>MSRAAQLLP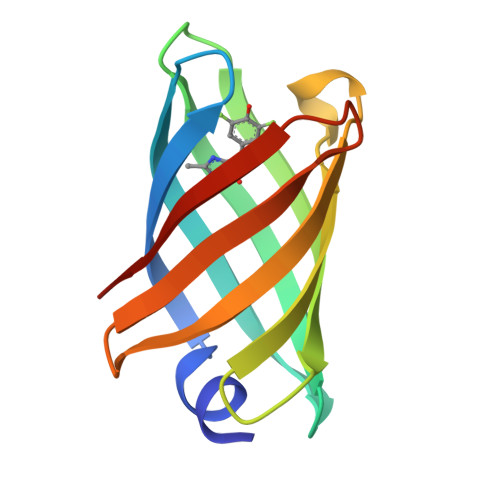GTWQVTMTNEDGQTSQGQWHFQPRSPYTLDIVAQGTISDGRPITGYGKATVKTDDTLHANLTYPSLGNIKAQGQITYDSPTQFTWNSTTSDGKKLTGTLQRQE[2x]> GAMEPPYFIEPLEHVEAAIGEPITLQCKVDGTPEIRIAWYKEHTKLRSAPAYKMQFKNNVASL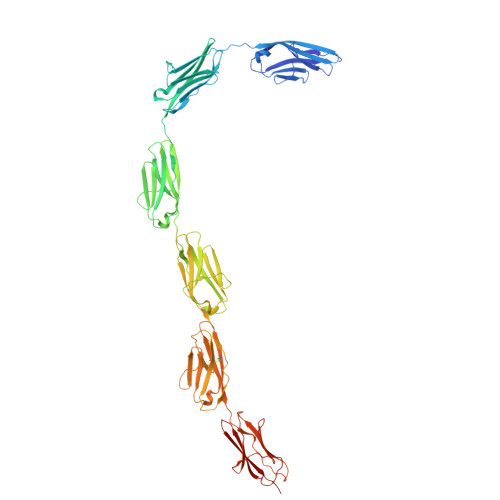VINKVDHSDVGEYTCKAENSVGAVASSAVLVIKERKLPPSFARKLKDVHETLGFPVAFECRINGSEPLQVSWYKDGELLKDDANLQTSFIHNVATLQILQTDQSHVGQYNCSASNPLGTASSSAKLTLSEHEVPPFFDLKPVSVDLALGESGTFKCHVTGTAPIKITWAKDNREIRPGGNYKMTLVENTATLTVLKVTKGDAGQYTCYASNVAGKDSCSAQLGVQEPPRFIKKLEPSRIVKQDEHTRYECKIGGSPEIKVLWYKDETEIQESSKFRMSFVESVAVLEMYNLSVEDSGDYTCEAHNAAGSASSSTSLKVKEPPVFRKKPHPVETLKGADVHLECELQGTPPFQVSWHKDKRELRSGKKYKIMSENFLTSIHILNVDSADIGEYQCKASNDVGSDTCVGSITLKAPPRFVKKLSDISTVVGEEVQLQATIEGAEPISVAWFKDKGEIVRESDNIWISYSENIATLQFSRAEPANAGKYTCQIKNEAGTQECFATLSVLE1-[2-(thiophen-2-yl)-1,3-thiazol-4-yl]methanamine 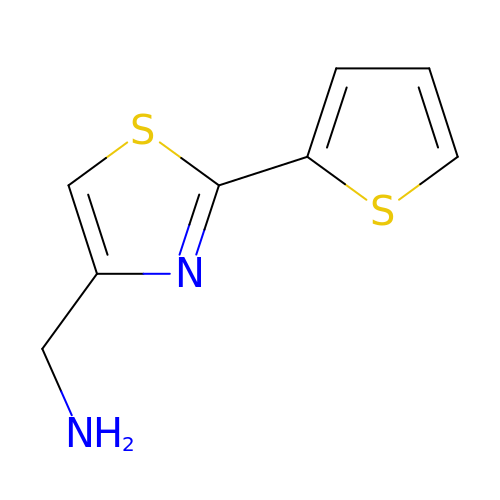| C8 H8 N2 S2 | VZBJIPJKJKKWPH-UHFFFAOYSA-N>[6x]GAMSCVYAFGSNGQRQLGLGHDEDMDTPQRSVPGDDGAIVRKIACGGNHSVMLTNDGNLVGCGDNRRGELDSAQALRQVHDWRPVEVPAPVVDVACGWDTTVIVDADGRVWQRGGGCYEFTQQHVPLNSNDERIAVYGCFQNFVVVQGTRVYGWGSNTKCQLQEPKSRSLKEPVLVYDTGSVAVDYVAMGKDFMVIVDEGGRIVHASGRL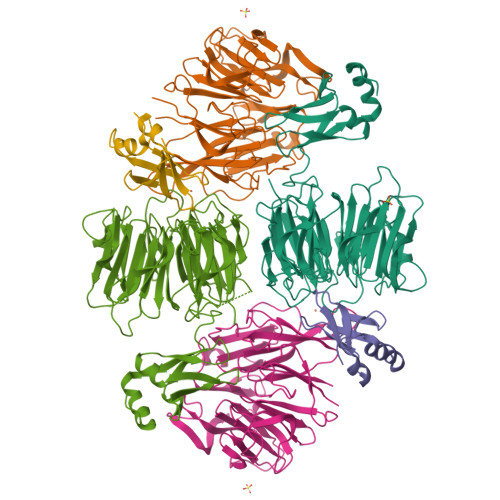PTGFELKQQQKRHNLVVLCMWTSIHLWNARLNTVESFGRGTHSQLFPQERLDFPIVGVATGSEHGILTTANQEGKSHCYNVYCWGWGEHGNCGPQKGSQPGLQLVGQYSGKPRVFGGCATTWIVLGSGSGSGSGSMSTYDEIEIEDMTFEPENQMFTYPCPCGDRFQIYLDDMFEGEKVAVCPSCSLMIDVVFDKEDLAEYYEEAGIHPPEPIAAAA>MSLCRWAAYHGTPIFLEDVISRPGHSLIAQSAHAEECKTATNGDGFGVAWYDARPEPGLYRDVYPAWSDPNLRAVAHHVRSGLFLSHVRASTGSCISRNNCHPFAARRWCFMHNGQVGGFEAFRKQADMAIADEFYTYRKGSTDSEVLFLLALSEGLEHDPHGALARAIARLEGLSRAHGTTPHMRLSAAFSDGQTLYAARYSSDHIAPSVYYRYSHARQGWAVVSEPLETDEGDWTELRPGR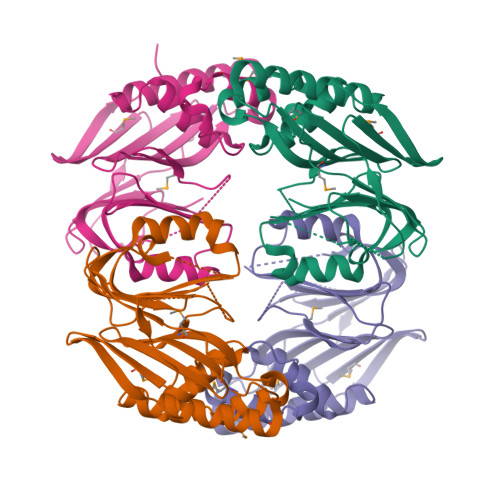MLTIGAEGAAERDFAPADLGRAAEGHHHHHH[4x]>[12x]HM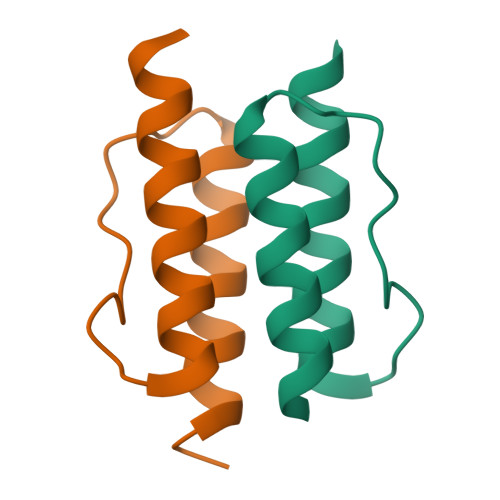STITRPIIELSNTVDKIAEGNLEAEVPHQNRADEIGILAKSIERLRRSLKVAME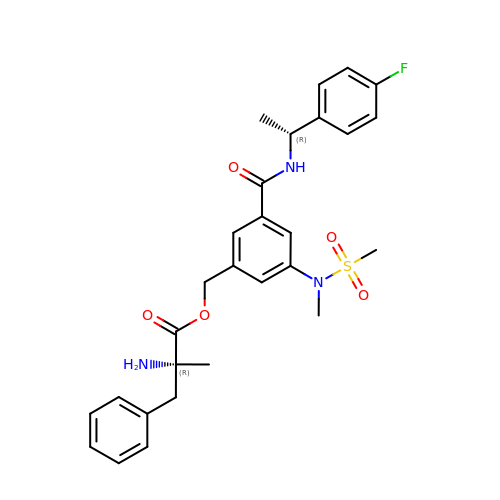3-({[(1R)-1-(4-FLUOROPHENYL)ETHYL]AMINO}CARBONYL)-5-[METHYL(METHYLSULFONYL)AMINO]BENZYL ALPHA-METHYL-D-PHENYLALANINATE | C28 H32 F N3 O5 S | PTQRJCCBUDSHTQ-WHLCRQNOSA-N> GGGGUGUGCCCGGCAUGGGUGCAGUCUAUAGGGUGAGAGUCCCGAACUGUGAAGGCAGAAGUAACAGUUAGCCUAACGCAAGGGUGUCCGUGGCGACAUGGAAUCUGAAGGAAGCGGACGGCAAACCUUCGGUCUGAGGAACACGAACUUCAUAUGAGGCUAGGUAUCAAUGGAUGAGUUUGCAUAACAAAACAAAGUCCUUUCUGCCAAAGUUGGUACAGAGUAAAUGAAGCAGAUUGAUGAAGGGAAAGACUGCAUUCUUACCCGGGGAGGUCUGGAAACAGAAGUCAGCAGAAGUCAUAGUACCCUGUUCGCAGGGGAAGGACGGAACAAGUAUGGCGUUCGCGC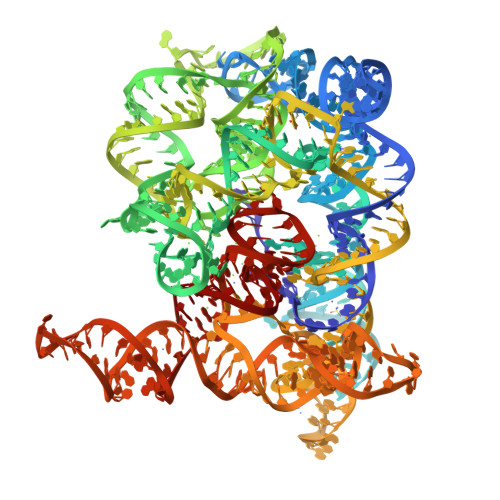CUAAGCUUGAACCGCCGUAUACCGAACGGUACGUACGGUGGUGUG> MEWSQIFHDITTKHDFKAMHDFLEKEYSTAIVYPDRENIYQAFDLTPFENIKVVILGQDPYHGPNQAHGLAFSVQPNAKFPPSLRNMYKELADDIGCVRQTPHLQDWAREGVLLLNTVLTVRQGEANSHRDIGWETFTDEIIKAVSDYKEHVVFILWGKPAQQKIKLIDTSKHCIIKSVHPSPLSAYRGFFGSKPYSKANTYLESVGKSPINWCESEALEHHHHHH;> MKQIKAHLTRYLEEILKLSSQEYLTEFVQLGIEELAWGERKIPEKLKGAIIDTYTFYDHSLIKDYIYSFIGTYQGKIILVGYTNGEYEHFFYINDTVKTLHSELHLLNLTEEDLEFVNVG

Ung (family 1 of the UDG superfamily) is the most prevalent form of UDG and removes uracil bases, regardless of their state of base pairing or sequence context, via the cleavage of the glycosyl bond attaching them to the deoxyribose. Ung inhibitors (which are interchangeably referred to herein as UngIns) are DNA mimetic proteins utilising charge-based alignment with the Ung DNA binding cleft to dock Ung. Docking promotes the hydrophobic sequestration of the sidechain of the apical residue in the Ung DNA minor groove binding loop, which is essentially irreversible under biological conditions, to inhibit Ung. UngIn protein structures described to date fall into one of three observed folds: Ugi/SAUGI (note that Ugi and SAUGI share the same protein fold at ~12% sequence residue identity), p56, and Vpr; yet, within each fold, type there is pronounced sequence plasticity, to the extent that the unambiguous identification of an Ung inhibitor in any genome is rarely straightforward.

The sequences MCUGI1, MCUGI2, MBUGI, SYUGI, and JMUGI were biochemically validated to act as UngIns; the sequence MCUGI1 was also structurally validated to act as an UngIn by co-crystallisation with SAUNG. The structural conservation between SAUGI and MCUGI1 variants is observed to be close with RMSD = 1.005 Å at low levels of sequence identity (29%). SAUGI contains 17 acidic residues, while MCUGI1 has 18 acidic residues. Just five such positions of negative charge are common to both sequences, of which, three are located within a 10-residue span in the Ung-binding β-strand 1 and α-helix 2. Of eight residues comprising the Ung binding β-strand, 24ECESIEEI31 in SAUGI and 24LTEFVQLG31 in MCUGI1, only a single glutamic acid residue is common to these variants and five residues comprise non-conservative variation. The Ung-sequestering hydrophobic pocket of SAUGI is formed by six residues, of which, only three are identical in MCUGI1. The other three residues forming the hydrophobic pocket in MCUGI1 do not align either at the sequence or structure level with those forming the hydrophobic pocket in the prototypical SAUGI, although residue side chains do occupy the same position in space. The surface negative charge distribution of MCUGI1 is somewhat different to that in Ugi, Ugi-2, and SAUGI. However, common properties among all these four Ugi/SAUGI variants include an invariant glutamic acid residue, a conserved acidic motif, and a spatially conserved hydrophobic pocket.>LLPVKYCKMRIFSGST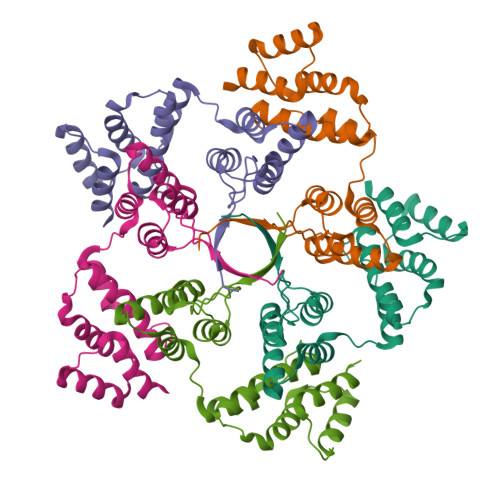AAAPEEEPFEVWLEQATEIAKEWPIPEAEKKRWVAESLRGPALDLMHIVQADNPSISVGECLEAFKQVFGSTESRRTSQVKYLRTYQQEGEKISAYVLRLETLLRRAVEKRAIPRNIADQVRLEQVMAGANLGNVLWCRLQELKDQGPLPTFLQLMKVIREEEE[5x]> GPLGSEDELYRQSLEIISRYLREQATGAKDTKPMGRSGATSRKALET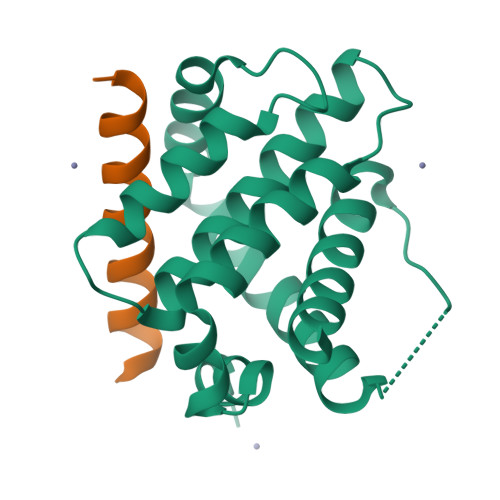LRRVGDGVQRNHETAFQGMLRKLDIKNEDDVKSLSRVMIHVFSDGVTNWGRIVTLISFGAFVAKHLKTINQESCIEPLAESITDVLVRTKRDWLVKQRGWDGFVEFFHVEDLEGG;> DMRPEIWIAQELRRIGDEFNAYYARR> SSGSSYPSLLQCLKAPVLSNSSCKSSYPGQITGNM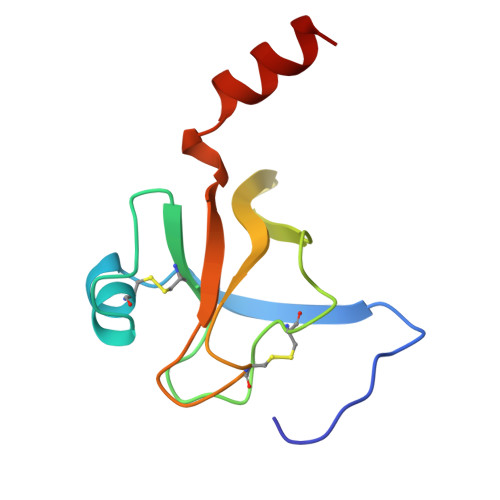ICVGFLQGGKDSCQGDSGGPVVCNGQLQGIVSWGYGCAQKNKPGVYTKVCNYVNWIQQTIAAN>[8x]MQYKKIITSESVGAGHPDKICDQISDAILDECLSQDQNSRVACEVLACNRLIVIAGEITTHAYVDVVKTAWEIIKPLGYDENDFTIISNVNK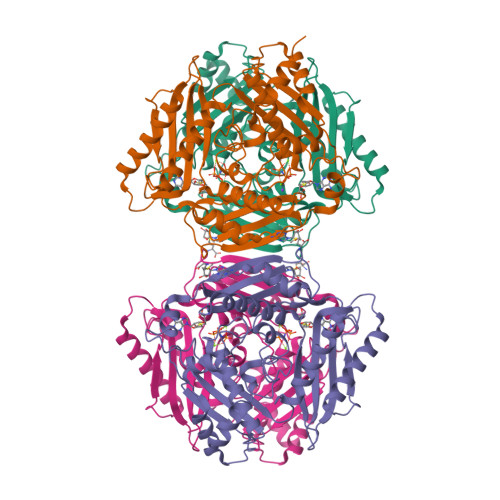QSVDIAQSVDKTNKNLIGAGDQGIVFGYACDETPQYMPLTSVLAHELLKEIERQRRSKEFIKIQADMKSQVSIDYSNSTPLIETMLVSIQHDEDYDVEYFNKKVSAIMEQIAKKYNLNTNFKKIINSSGRFVIGGPIGDTGLTGRKIIVDTYGGVGHHGGGAFSGKDPTKVDRSASYFARWIAKNVVAAKLAKQCEIQLAFAIGQPQPVAMYVNTFNTNLIDETKIFEAIKKSFNFDIKTFINDLNLWTTKYLPVATYGHFGRDDLDLSWEKLNKVEDLIKNSKHHHHHH>MKTMRKQIYKKAYWLLLPFLPLALANTFLVKEDSKNVTAYTPFATPITDSKSDLVSLAQLDSSYQIADQTIHNTNLFVLFKSRDVKVKYESSGSNNISFDSTSQGEKPSYVVEFTNSTNIGIKWTMVKKYQLDVPNVSSDMNQVLKNLILEQPLTKYTLNSSLAKEKGKTQREVHLGSGQANQWTSQRNQHDLNNNPSPNASTGFKLTTGNAYRKLSESWPIYEPIDGTKQGKGKDSSGWSSTEENEAKNDAPSVSGGGSSSGTFNKYLNTKQALESIGILFDDQTPRNVITQLYYASTSKLAVTNNHIVVMGNSFLPSMWYWVVERSAQENASNKPTWFANTNLDWGEDKQKQFVENQLGYKETTSTNSHNFHSKSFTQPAYLISGIDSVNDQIIFSGFKAGSVGYDSSSSSSSSSSSSTKDQALAWSTTTSLDSKTGYKDLVTNDTGLNGPINGSFSIQDTFSFVVPYSGNHTNNGTTGPIKTAYPVKKDQKSTVKINSLINATPLNSYGDEGIGVFDALGLNYNFKSNQERLPSRTDQIFVYGIVSPNELRSAKSSADSTGSDTKVNWSNTQSRYLPVPYNYSEGIIDADGFKRPENRGASVTTFSGLKSIAPDGFANSIANFSVGLKAGIDPNPVMSGKKANYGAVVLTRGGVVRLNFNPGNDSLLSTTDNNIAPISFSFTPFTAAESAVDLTTFKEVTYNQESGLWSYIFDSSLKPSHDGKQTPVTDNMGFSVITVSRTGIELNQDQATTTLDVAPSALAVQSGIQSTTQTLTGVLPLSEEFSAVIAKDSDQNKIDIYKNNNGLFEIDTQLSNSVATNNGGLAPSYTENRVDAWGKVEFADNSVLQARNLVDKTVDEIINTPEILNSFFRFTPAFEDQKATLVATKQSDTSLSVSPRIQFLDGNFYDLNSTIAGVPLNIGFPSRVFAGFAALPAWVIPVSVGSSVGILFILLVLGLGIGIPMYRVRKLQDASFVNVFKKVDTLTTAVGSVYKKIITQTGVVKKAPSALKAANPSVKKPAAFLKPPVQPPSKPEGEQKAVEVKSEETKS[2x];>MHQPKKRLAKKSWAFLTAALTLGVITGVGGYFLFNQNKQRSSVSNFAYQPKQLSVKHQQAVDETLTPWTWNNNNFSSLKITGENPGSFGLVRSQNDNLNISSVTKNSSDDNLKYLNAVEKYLDGQQNFAIRRYDNNGRALYDINLAKMENPSTVQRGLNGEPIFDPFKGFGLTGNAPTDWNEIKGKVPVEVVQSPHSPNLYFVLLVPKVALEYHNLNNQVVKESLEVKATQSSFNPTQRLQKDSPVKDSSKQGEKLSETTASSMSSGMATSTRAKALKVEVERGSQSDSLLKNDFAKKPLKHKNSSGEVKLEAEKEFTEAWKPLLTTDQIAREKGMGATVVSFYDAPYSENHTAFGLVDHIDPKKMVENYPPSWKTPKWNHHGIWDYNARNLLLQTTGFFNPRRHPEWFDEGQAKADNTSPGFKVGDTDHKKDGFKKNSSSPIALPFEAYFANIGNMVAIGNSVFIFGGNGHATKMFTTNPLSIGVFRIKYTDNFSKSSVTGWPYAVLFGGLINPQTNGLKDLPLGTNRWFEYVPRMAVSGVKWVGNQLVLAGTLTMGDTATVPRLKYDQLEKHLNLVAQGQGLLREDLQIFTPYGWANRPDIPVGAWLQDEMGSKFGPHYFLNNPDIQDNVNNDTVEALISSYKNTDKLKHVYPYRYSGLYAWQLFNWSNKLTNTPLSANFVNENSYAPNSLFAAILNEDLLTGLSDKIFYGKENEFAENEADRFNQLLSLNPNPNTNWARYLNVVQRFTTGPNLDSSTFDQFLDFLPWIGNGKPFSNSPSPSTSASSSTPLPTFSNINVGVKSMITQHLNKENTRWVFIPNFSPDIWTGAGYRVQSANQKNGIPFEQVKPSNNSTPFDPNSDDNKVTPSGGSSKPTTYPALPNSISPTSDWINALTFTNKNNPQRNQLLLRSLLGTIPVLINKSGDSNDQFNKDSEQKWDKTETNEGNLPGFGEVNGLYNAALLHTYGFFGTNTNSTDPKIGFKADSSSSSSSTLVGSGLNWTSQDVGNLVVINDTSFGFQLGGWFITFTDFIRPRTGYLGITLSSLQDQTIIWADQPWTSFKGSYLDSDGTPKSLWDPTALKSLPNSSTTYDTNPTLSPSFQLYQPNKVKAYQTTNTYNKLIEPVDATSAATNMTSLLKLLTTKNIKAKLGKGTASSQGNNNGGGVSQTINTITTTGNISEGLKEETSIQAETLKKFFDSKQNNKSEIGIGDSTFTKMDGKLTGVVSTPLVNLINGQGATSDSDTEKISFKPGNQIDFNRLFTLPVTELFDPNTMFVYDQYVPLLVNLPSGFDQASIRLKVISYSVENQTLGVRLEFKDPQTQQFIPVLNASSTGPQTVFQPFNQWADYVLPLIVTVPIVVIILSVTLGLTIGIPMHRNKKALQAGFDLSNKKVDVLTKAVGSVFKEIINRTGISNAPKKLKQATPTKPTPKTPPKPPVKQ[2x]

The nap particle is an immunogenic surface adhesion complex from Mycoplasma genitalium. It is essential for motility and responsible for binding sialylated oligosaccharides on the surface of the host cell. Cryo-electron tomography (cryo-ET) of M. genitalium revealed the tetrameric organization of the nap particle complex, consisting of two P140-P110 heterodimers. The P140-P110 heterodimers form the ‘tight interface’, while the ‘loose interface’ is formed between the two heterodimers.

Here, we determined the structure of the complete native nap particle complex in-situ, including the previously uncharacterized intracellular region at 11 Å resolution using cryo-ET. In the cryo-ET reconstructions, the entire nap particle including the intracellular domain can be seen, displaying a highly electron dense and structured region (white arrow). The density of the previously unresolved intracellular region was solved at 11 Å resolution, thereby providing a model of the entire nap particle. The previously uncharacterized intracellular region appears compact proximal to the membrane and forms two distinct branches distal to the membrane. The previously uncharacterized residues 937–1053 of P110 and 1348–1444 of P140 were predicted with high confidence using Alphafold as a four-helix bundle splitting into two-helix branches. The Alphafold model could be fitted into the density of the intracellular region using rigid body docking. The transmembrane region forms a ~40-residue four-helix bundle proximal to the membrane and an unstructured flexible loop (predicted with low confidence and therefore not displayed) distal to the membrane of approximately 36 and 28 amino acids for P110 and P140, respectively. The intracellular density measures ~90 Å along the symmetry axis of the nap particle, being ~50 Å wide at the distal end, with 5 Å between the two branches. The density allows for the docking of all four intracellular helices, showing that residues from P110 are likely to form the distal branch of the intracellular density. The residues 1017–1053 of P110 and 1416–1444 of P140 were predicted with little confidence as an unstructured loop and are not displayed in this model.>[4x]MAEIPKEMLRAQTNVILLNVLKQGDNYVYGIIKQVKEASNGEMELNEATLYTIFKRLEKDGIISSYWGDESQGGRRKYYRLTEIGHE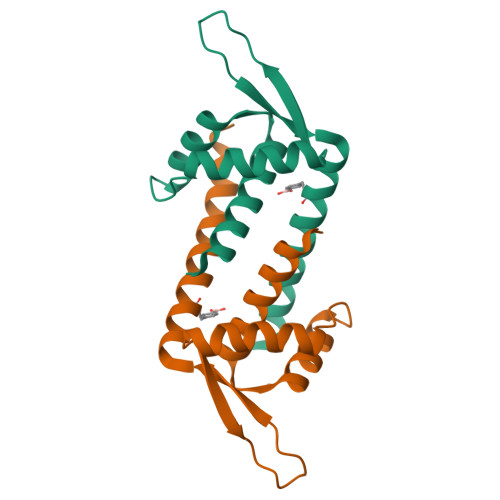NFRLAFESWSRVDKIIENLEANKKSEAIKSRWSHPQFEK>APADNAADARPVDVSVSIFINKIYGVNTLEQTYKVDGYIVAQWTGKPRKTPGDKPLIVENTQIERWINNGLWVPALEFINVVGSPDTGNKRLMLFPDGRVIYNARFLGSFSNDMDFRLFPFDRQQFVLELEPFSYNNQQLRFSDIQVYTENIDNEEIDEWWIRGKASTHISDIRYDHLSSVQPNQNEFSRITVRIDAVRNPSYYLWSFILPLGLIIAASWSVFWLESFSERLQTSFTLMLTVVAYAFYTSNILPRLPYTTVIDQMIIAGYGSIF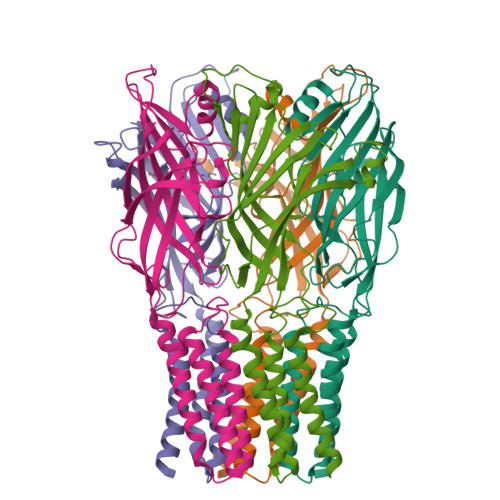AAILLIIFAHHRQANGVEDDLLIQRCRLAFPLGFLAIGCVLVIRGITL[5x]>MENFPTEYFLNTTVRLLEYIRYRDSNYTREERIENLHYAYNKAAHHFAQPRQQQLLKVDPKRLQASLQTIVGMVVYSWAKVSKECMADLSIHYTYTLVLDDSKDDPYPTMVNYFDDLQAGREQAHPWWALVNEHFPNVLRHFGPFCSLNLIRSTLDFFEGCWIEQYNFGGFPGSHDYPQFLRRMNGLG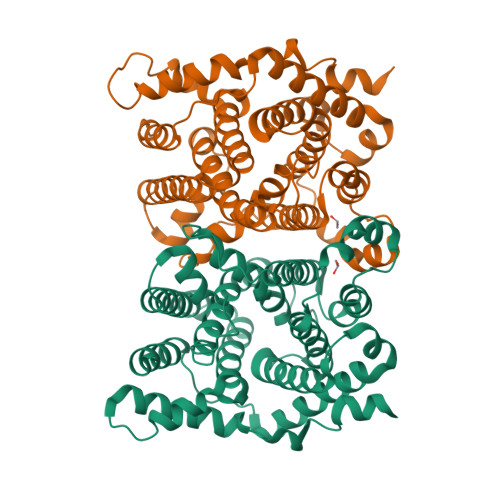HCVGASLWPKEQFNERSLFLEITSAIAQMENWMVWVDDLMTFYKEFDDERDQISLVKNYVVSDEISLHEALEKLTQDTLHSSKQMVAVFSDKDPQVMDTIECFMHGYVTWHLCDRRYRLSEIYEKVKEEKTEDAQKFCKFYEQAANVGAVSPSEWAYPPVAQLANVRSKDVKEVQKPFLSSIELVE[2x]>NSPTMVIMVGLPARGKTYISTKLTRYLNFIGTPTKVFNLGQYRREAVSYKNYEFFLPDNMEALQIRKQCALAALKDVHNYLSHEEGHVAVFDATNTTRERRSLILQFAKEHGYKVFFIESICNDPGIIAENIRQVKLGSPDYIDCDREKVLEDFLKRIECYEVNYQPLDEELDSHLSYIKIFDVGTRYMVNRVQDHIQSRTVYYLMNIHVTPRSIYLCRHGESELNIRGRIGGDSGLSVRGKQYAYALANFIQSQGISSLKVFTSRMKRTIQTAEALGVPYEQFKALNEIDAGVCEEMTYEEIQEHYPEEFALR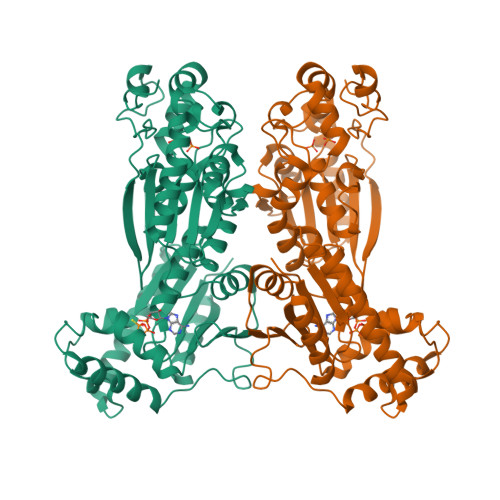DQDKYRYRYPKGESYEDLVQRLEPVIMELERQENVLVICHQAVMRCLLAYFLDKSSEELPYLKCPLHTVLKLTPVAYGCKVESIYLNVEAVNTHREKPENVDITREPEEALDTVPAHY[2x]[[(2R,3S,5R)-5-[5-methyl-2,4-bis(oxidanylidene)pyrimidin-1-yl]-3-oxidanyl-oxolan-2-yl]methoxy-oxidanyl-phosphoryl] [(2R,3R,4S,5R,6R)-6-methyl-3,4,5-tris(oxidanyl)oxan-2-yl] 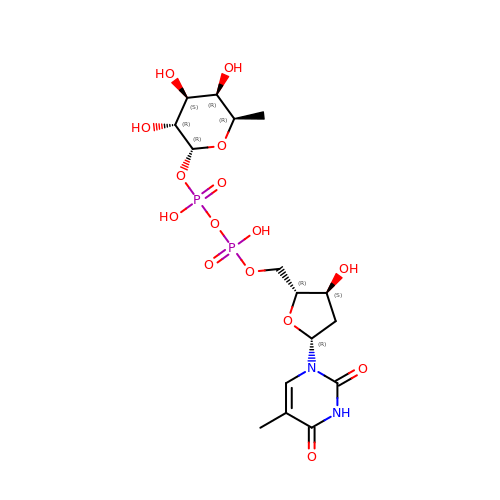hydrogen phosphate | C16 H26 N2 O15 P2 | ZOSQFDVXNQFKBY-FQLHZTMTSA-N>KASAAKAGDILLSHSFEEGTTQGWTARGGVKVDVTAEQAYQGKQSLQTTGRTEAWNGPSLSLTDVVHKNEVVEISGYVKLVAGSAPADLKFTVERRDGNGDTQYDQVNAAEQVTDQKWVKLQGQYSYEQGSSLLLYLESTDAKAAYLLDEFQIRLVKAAPENPGEPGEAGQALFKADFEDGNIGNWRARGTEKLEVVSGIGHNSNRSLKTSSRSETYHGPLVEVLPYLQKGSTVHISFWAMYDEGPATQVINGSLEKEFNRDTANLEYAMFASTTLNKGQWKKIEADIIVPAESTGISGLRMYAETPWKQSSEVTETDTIPFY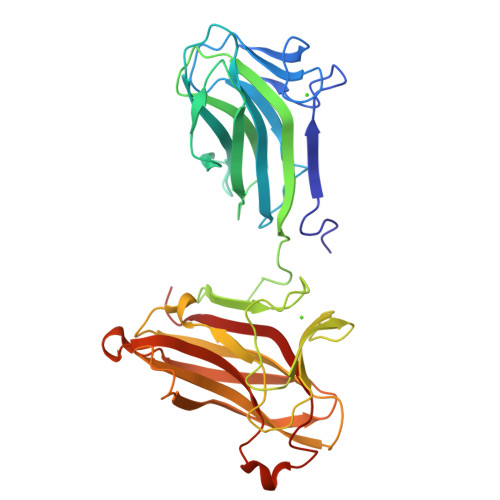VDDVQITATEA[6x]> MPISPIETVPVKLKPGMDGPKVKQWPLTEEKIKALVEICTEMEKEGKISKIGPENPYNTPVFAIKKKDSTKWRKLVDFRELNKRTQDFWEVQLGIPHPAGLKKKKSVTVLDVGDAYFSVPLDEDFRKYTAFTIPSINNETPGIRYQYNVLPQGWKGSPAISQSSMTKILEPFKKQNPDIVIYQYMDDLYVGSDLEIGQHRTKIEELRQHLLRWGLTTPDKKHQKEPPFLWMGYELHPDKWTVQPIVLPEKDSWTVNDIQKLVGKLNWASQIYPGIKVRQLSKLLRGTKALTEVIPLTEEAELELAENREILKEPVHGVYYDPSKDLIAEIQKQGQGQWTYQIYQEPFKNLKTGKYARMRGAHTNDVKQLTEAVQKITTESIVIWGKTPKFKLPIQKETWETWWTEYWQATWIPEWEFVNTPPLVKLWYQLEKEPIVGAETFY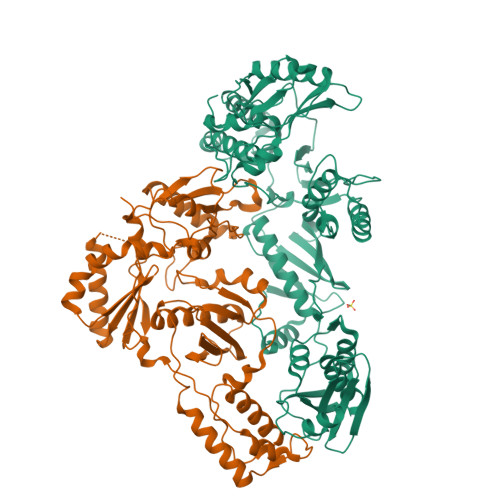VDGAANRETKLGKAGYVTNKGRQKVVPLTNTTNQKTELQAIYLALQDSGLEVNIVTDSQYALGIIQAQPDKSESELVNQIIEQLIKKEKVYLAWVPAHKGIGGNEQVDKLVSAG;> ETVPVKLKPGMDGPKVKQWPLTEEKIKALVEICTEMEKEGKISKIGPENPYNTPVFAIKKKDSTKWRKLVDFRELNKRTQDFWEVQLGIPHPAGLKKKKSVTVLDVGDAYFSVPLDEDFRKYTAFTIPSINNETPGIRYQYNVLPQGWKGSPAIFQSSMTKILEPFKKQNPDIVIYQYMDDLYVGSDLEIGQHRTKIEELRQHLLRWGLTTPDKKHQKEPPFLWMGYELHPDKWTVQPIVLPEKDSWTVNDIQKLVGKLNWASQIYPGIKVRQLSKLLRGTKALTEVIPLTEEAELELAENREILKEPVHGVYYDPSKDLIAEIQKQGQGQWTYQIYQEPFKNLKTGKYARMRGAHTNDVKQLTEAVQKITTESIVIWGKTPKFKLPIQKETWETWWTEYWQATWIPEWEFVNTPPLVKLWYQ>TWDIPDLFINTCGASGFEQPQNCDHNRELDGQTGHFLKEDGTQQWTVPVTGFYRMEICGAGGGSNSKASGDTGDCVTLQVHLIENLSLRMLIGQMGESPCFTEHDDELRPSSCSKISHNYVYDGKRGAAGGGATLLTVEKDLWNVVAGGGAGASWDGFDMEVGYGASAIHVKPDQRCNETCKAVSHTDFIVERRDNRCPGEKGESTVFGGFGGGGNSCGMLGGSGAGYQAGNPFGKSR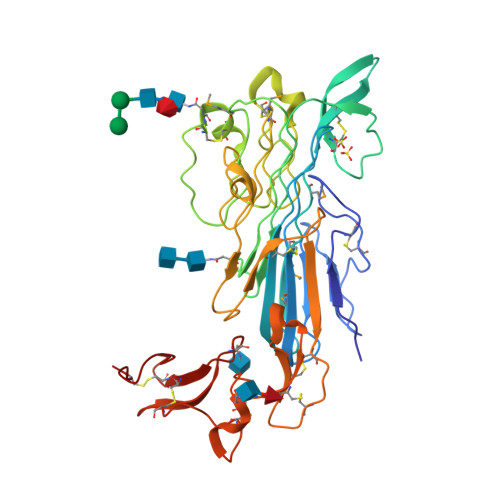ARSGSSNVSIDFSKSPIYYQSERLDEGYIKIAFCRKRCEPPTVCRFRKDYFEEEYCGCPDGSNVTDTEEACAFPLVCPSSSTNQYRNFTYEPFCLCNNGKEIYDVYNDTCEE[2x]>[2x]SNAMPLPKSLKYGDTIGIYSPSSPVTYTSPKRFERAKSYLLQKGFHILEGSLTGRYDYYRSGSIQERAKELNALIRNPNVSCIMSTIGGMNSNSLLPYIDYDAFQNNPKIMIGYSDATALLLGIYAKTGIPTFYGPALVPSFGEFEPFVDDTYKYFLETLLHDQALPYNIKQPLFWSDESINWEEKTKEKELRPNNWISVT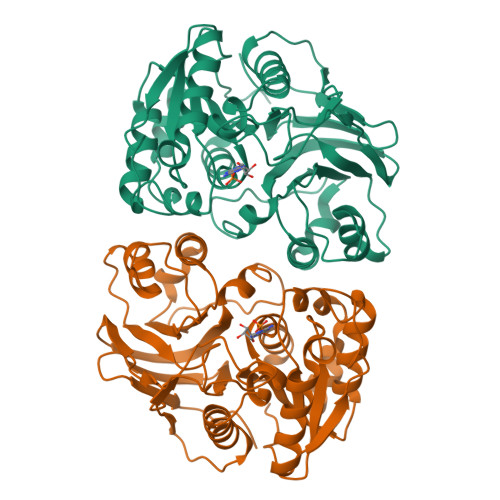NGQATGRVIGGNLNTIQGIWGSPYMPCIQEGDILFIEDSSKDAATIERSFSFLKINGVFDKVSGIILGKHEQFDDCGTNRKPYEILLEVLQNQRIPLLADFDCCHTHPMITMPIGVQVKMDATNKTIHILEKWKI4-[[3-[2-chloranyl-6-(trifluoromethyl)phenyl]-5-(1~{H}-pyrrol-3-yl)-1,2-oxazol-4-yl]methoxy]benzoic acid | C22 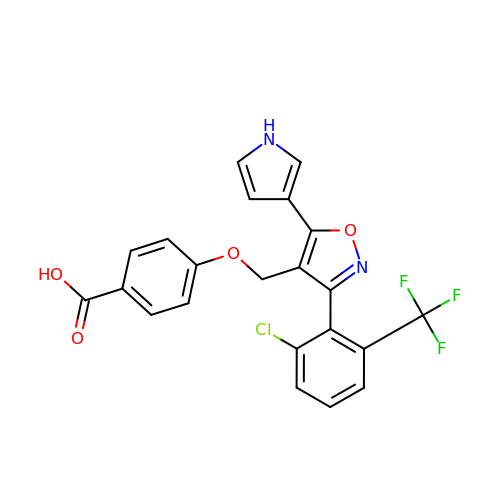H14 Cl F3 N2 O4 | NZRBQNXUTCVFCO-UHFFFAOYSA-N>MGSSHHHHHHSSGLVPRGSHMSNVKDMSLAPSGHLKMEWAKRHMPVLCRIAEEFKNDKPFEGLTIGMALHLEAKTAILAETLLEGGAKIVITGCNPLSTQDDVAAACVEKGMEVYAWRGETNEEYYENLNKVLDSNPDIIIDDGADLIFLIHTERTELIGKIMGGCEETTTGIIRLKSMAEEGALKFPVVNVNDAYTKHLFDNRYGTGQSAMDGIIRTTNLLIAGKNVVVGGYGWCGRGVASRAAGHGANVIITEVNPIRALEAKMDGFTVLKMEEAAKIGDIFVTTTGCKDILRMEHFLLMKDGAVLSNAGHFDNEINKNDLKELSKSVKEARFNIEEYDLGNKKIYLLGEGRLVNLACADGHPCEVMDMSFANQALSAKFIKENKGKLENEVY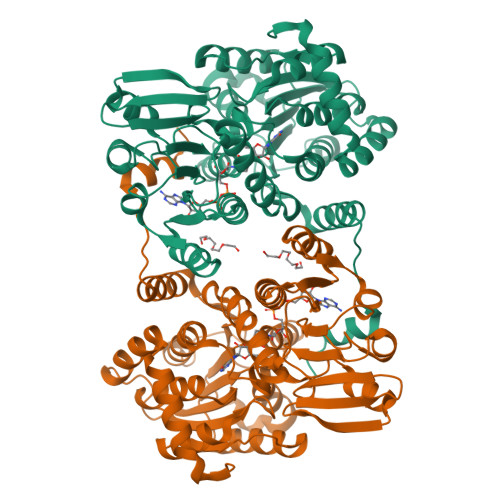EIPYEQDFKIALLKLHSMGADIDELSPEQRKYLSDWKEGT[8x]> MPIATPEVYAEMLGQAKQNSYAFPAINCTSSETVNAAIKGFADAGSDGIIQFSTGGAEFGSGLGVKDMVTGAVALAEFTHVIAAKYPVNVALHTDHCPKDKLDSYVRPLLAISAQRVSKGGNPLFQSHMWDGSAVPIDENLAIAQELLKAAAAAKIILEIEIGVVGGEEDGVANEINEKLYTSPEDFEKTIEALGAGEHGKYLLAATFGNVHGVYKPGNVKLRPDILAQGQQVAAAKLGLPADAKPFDFVFH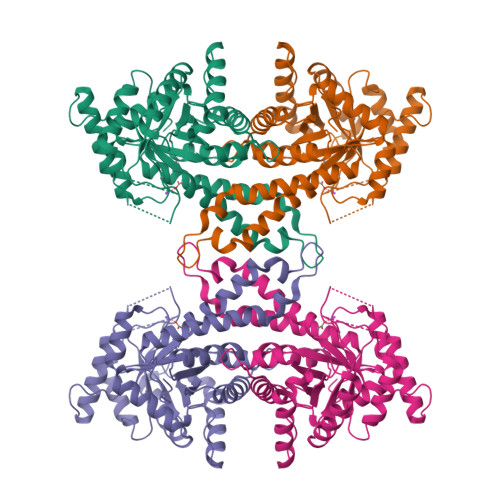GGSGSLKSEIEEALRYGVVKMNVDTDTQYAFTRPIAGHMFTNYDGVLKVDGEVGVKKVYDPRSYLKKAEASMSQRVVQACNDLHCAGKSLTHHHHHH>EKTCDL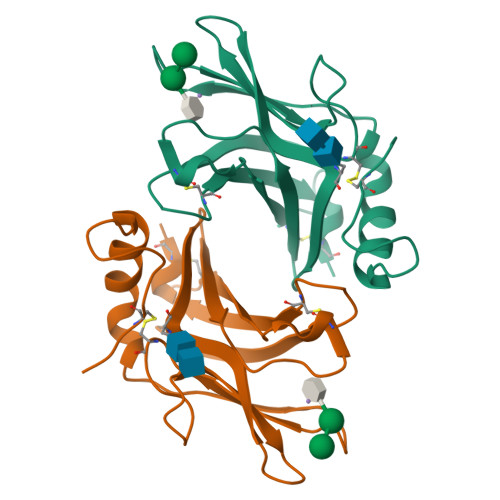VGEKGKESEKELALLKRLTPLFQKSFESTVGQSPDMYSYVFRVCREAGQHSSGAGLVQIQKSNGKETVVGRFNETQIFQGSNWIMLIYKGGDEYDNHCGREQRRAVVMISCNRHTLADNFNPVSEERGKVQDCFYLFEMDSSLACS[2x]> MQRTLRSLATRCAGAITGSTAQTGASGCIKAEAGVSTSALSGLISQDAIHGLCPRGAAFASLASSGVSAAAGAGPASQLRAGAPLSCLWLLALAPSRTGLAATASSSSSCGACGSHSSTSSPFAPLPASAAGLRHYAKAAKGGAAAAPAAPSGPKRPRTSTTKLYSCRNDRLRHTHEQIWPTLQLTEYEQAMFK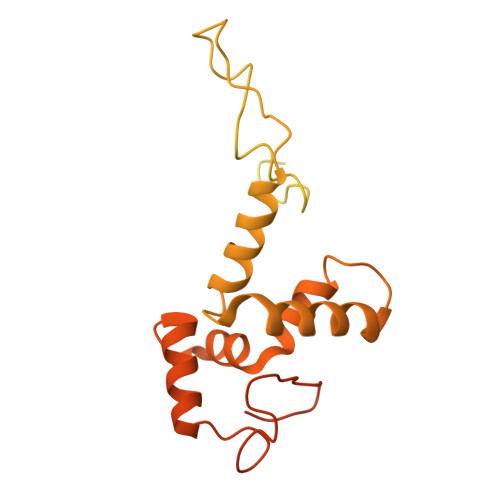RNSRLFVVDMGRSLSLRDKFRMGAYEPATAASTGAAAEEAGGAGAGDALVPAAGGASYRRVPYWQARSLLHESNLHLDALGENPRYLRLRRVGSLFATKLQNVRKLRLLLGFQRRGFVQKLYEHSLLARGSDRMWKMVCAMEATLPMTVTRMGLAEDVVGAATAIRNDKIYVNGKQPVMPRKGLLEPGDVVGPAAGGAAYLRKRVARSMEPLASVVTRDYV> GADSCKYCLQLYDET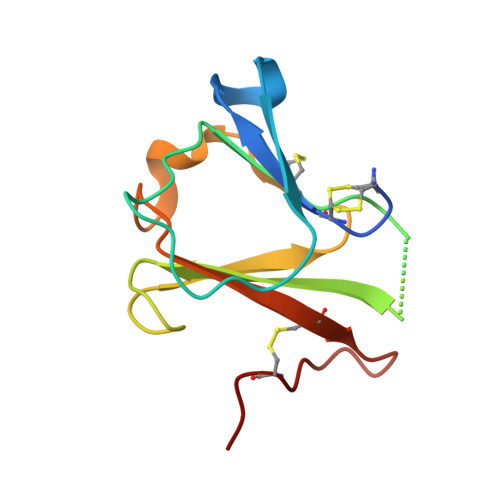YERGSYIEVYKSVGSLSPPWTPGSVCVPFVNDTKRERPYWYLFDNVNYTGRITGLGHGTCIDDFTKSGFKGISSIKRCIQTKDGKVECINQ N-(5,5-dioxodibenzothiophen-2-yl)-4,4-difluoro-piperidine-1-carboxamide 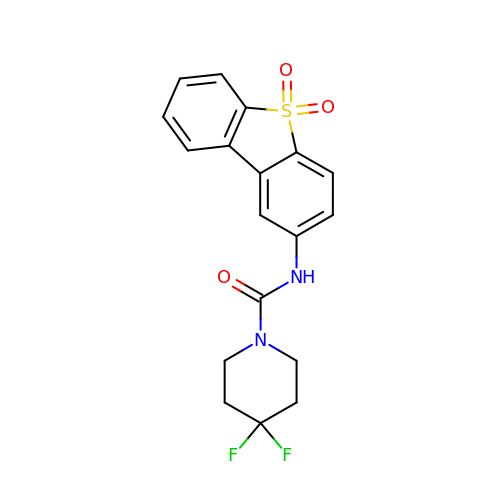| C18 H16 F2 N2 O3 S | CHISZLOVTPVOGH-UHFFFAOYSA-N>MAEKPKLHYFNGRGRMESTRWLLAAAGVEFEEKFIKSAEDLDKLRNDGYLMFQQVPMVEIDGMKLVQTRAILNYIASKYNLYGKDIKERALIDMYIEGIADLGEMIIMLPFCPPEEKDAKLALIKEKIKNRYFPAFEKVLKSHGQDYLVGNKLSRADIHLVELLYYVEELDSSLISSFPLLKALKTRISNLPTVKKFLQPGSPRKPPPDEIYVRTVYNIFRP[8x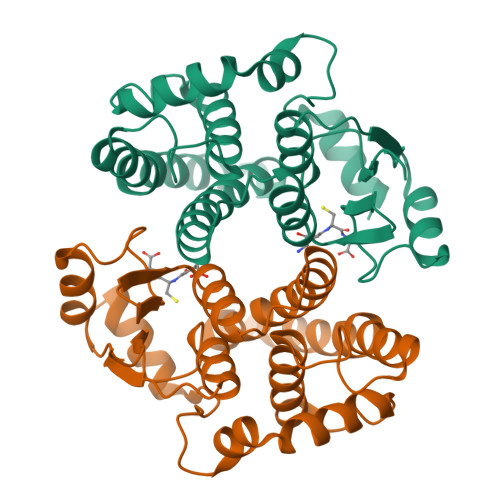]6-AMINO-4-[2-(4-METHOXYPHENYL)ETHYL]-1,7-DIHYDRO-8H-IMIDAZO[4,5-G]QUINAZOLIN-8-ONE | C18 H17 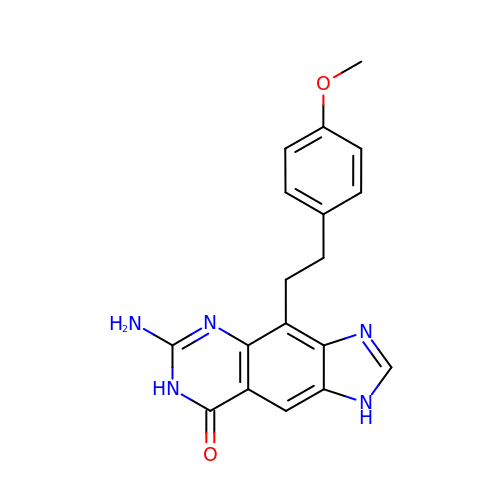N5 O2 | UKRVQKUVWNDGMN-UHFFFAOYSA-N>MEEHTQGSHVEAGIVEHPNAEDFGHARTLPTDTNWFKHAVFYEVLVRAFYDSNADGIGDLRGLTEKLDYIKWLGVDCLWLPPFYDSPLRDGGYDIRDFYKVLPEFGTVDDFVTLLDAAHRRGIRIITDLVMNHTSDQHEWFQESRHNPDGPYGDFYVWSDTSDRYPDARIIFVDTEESNWTFDPVRRQFYWHRFFSHQPDLNYDNPAVQEAMLDVLRFWLDLGIDGFRLDAVPYLFEREGTNCENLPETHAFLKRCRKAIDDEYPGRVLLAEANQWPADVVAYFGDPDTGGDECHMAFHFPLMPRIFMAVRRESRFPISEILAQTPPIPDTAQWGIFLRNHDELTLEMVTDEERDYMYAEYAKDPRMKANVGIRRRLAPLLENDRNQIELFTALLLSLPGSPVLYYGDEIGMGDIIWLGDRDSVRTPMQWTPDRNAGFSKATPGRLYLPPNQDAVYGY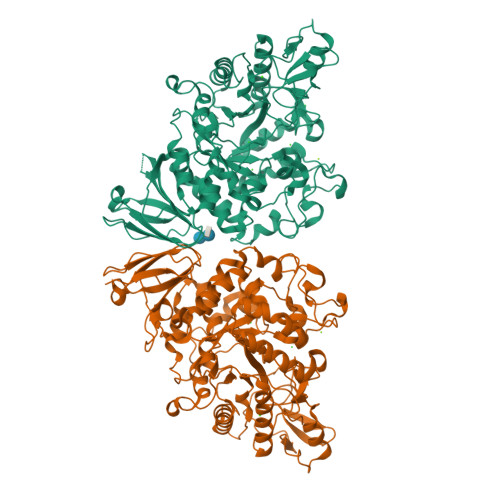HSVNVEAQLDSSSSLLNWTRNMLAVRSRHDAFAVGTFRELGGSNPSVLAYIREVTRQQGDGGAKTDAVLCVNNLSRFPQPIELNLQQWAGYIPVEMTGYVEFPSIGQLPYLLTLPGHGFYWFQLREPDPEPGAQQ[2x]>[6x]GNTVTIDFMSADGIVPGRTPVRYQGVEVGTVQDISLSDDLRK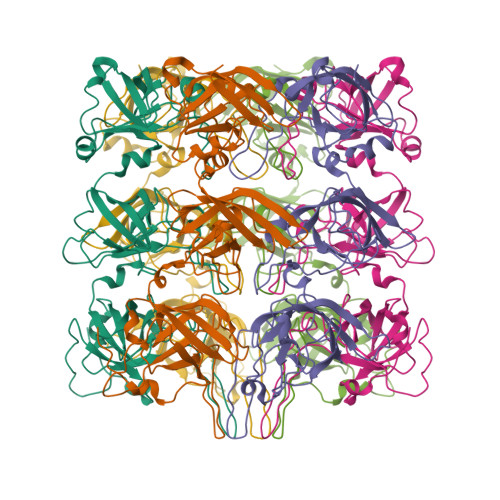IEVKVSIKSDMKDALREETQFWLVTPKASLAGVSGLDALVGGNYIGMMPGKGKEQDHFVALDTQPKYRLDNGDLMIHLQAPDLGSLNSGSLVYFRKIPVGKVYDYAINPNKQGVVIDVLIERRFTDLVKKGSRFWNVSGVDANVSISGAKVKLESLAALVNGAIAFDSPEESKPAEAEDTFGLYEDLAHSQRGVIIKLELPSGAGLTADSTPLMYQGLEVGQLTKLDLNPGGKVTGEMTVDPSVVTLLRENTRIELRNPKLSLSDANLSALLTGKTFELVPGDGEPRKEFVVVPGEKALLHEPDVLTLTLTAPESYGIDAGQPLILHGVQVGQVIDRKLTSKGVTFTVAIEPQHRELVKGDSKFVVNSRVDVKVGLDGVEFLGASASEWINGGIRILPGDKGEMKASYPLYANLEKALENSLSDLPTTTVSLSAETLPDVQAGSVVLYRKFEVGEVITVRPRANAFDIDLHIKPEYRNLLTSNSVFWAEGGAKVQLNGSGLTVQASPLSRALKGAISFDNLSGASASQRKGDKRILYASETAARAVGGQITLHAFDAGKLAVGMPIRYLGIDIGQIQTLDLITARNEVQAKAVLYPEYVQTFARGGTRFSVVTPQISAAGVEHLDTILQPYINVEPGRGNPRRDFELQEATITDSRYLDGLSIIVEAPEAGSLGIGTPVLFRGLEVGTVTGMTLGTLSDRVMIAMRISKRYQHLVRNNSVFWLASGYSLDFGLTGGVVKTGTFNQFIRGGIAFATPPGTPLAPKAQEGKHFLLQESEPKEWREWGTALPK> CMNKKNRLALRKRRRRMGERVS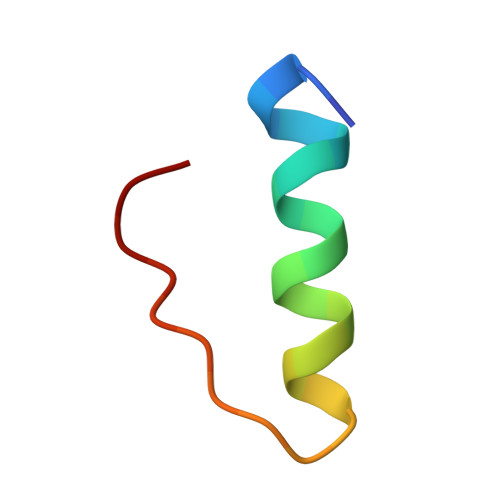LRYR(2R,3R,4S,5R,6S)-3-(acetylamino)-5-amino-4-hydroxy-6-methyltetrahydro-2H-pyran-2-yl 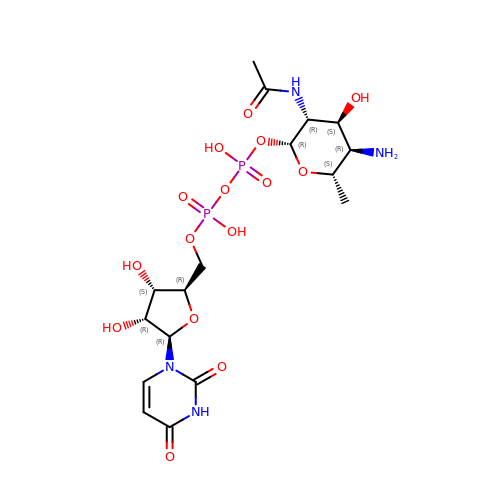[(2R,3S,4R,5R)-5-(2,4-dioxo-3,4-dihydropyrimidin-1(2H)-yl)-3,4-dihydroxytetrahydrofuran-2-yl]methyl dihydrogen diphosphate | C17 H28 N4 O15 P2 | FUUMLYWEEZBCQR-NAGKVERXSA-N>GSHMKPEIKEAYMKTAELFSQVSNCKRMKVGAIVVKNGSILAHGWNGTPSGFHTNCCELEDGSTNPFVLHAEQNALVKMAKSSESIDGSELFCTHSPCPDCSKMIAQAGVKKVYYRNE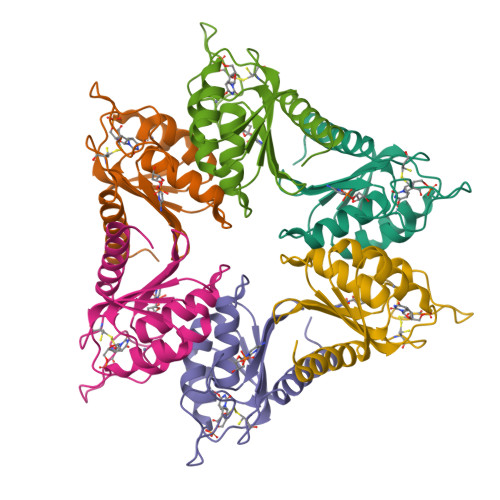YRITDGIDVLQQLGVEVEKM[12x]> SNAASGSALIFDEEMSRYKLLWTDPACEIEVPERLTVSYEALRTHGLAQRCKAVPVRQATEQEILLAHSEEYLEAVKQTPGMNVEELMAFSKKYNDVYFHQNIYHCAKLAAGATLQLVDSVMKREVRNGMALVRPPGHHSQRSAANGFCVFNNVAFAALYAKKNYNLNRILIVDWDVHHGQGIQYCFEEDPSVLYFSWHRYEHQSFWPNLPESDYSSVGKGKGSGFNINLPWNKVGMTNSDYLAAFFHVLLPVAYEFDPELVIVSAGFDSAIGDPEGEMCALPEIFAHLTHLLMPLAAGKMCVVLEGGFNLTSLGQSVCQTVHSLLGDPTPRISGLGTACDSALESIQNVRNVQSSYWSSFKHLAQSETNPKRPRLDATNGGPKESSEPASESNPKKTAQDIVWPEPLKRMPASVRTVVVPPPGVELTLPKNCQHSGDISESTAKEVQRIRDKHFHDLTDQNILRSLGNIISVLDRMMRSDEVCNGCVVVSDLSVSVQCALQHALTEPAERVLVVYVGDGELPVKTNDGKVFLVQICTKETEDKCVNRLTLCLREGESLTAGFMQALLGLILPVAYEFNPALVLGIVEETAAKTRLMRVWGHMTCLIQGLARGRMLTLLQGYDKDLLELTVSALSGASISPLGPLRAPKPEDVEMMEKQRQRLQERWGLLRCTVSESW

Here we report enzymological studies conclusively demonstrating that HDAC10 is a robust PDAC and a poor lysine deacetylase. Therefore, HDAC6 is clearly an acetyllysine deacetylase and HDAC10 is an N8-acetylspermidine deacetylase. In addition, we report the 2.85-Å resolution crystal structure of HDAC10 complexed with a polyamine transition state analogue inhibitor. This structure reveals that the conserved glutamate gatekeeper and a sterically constricted active site confer specificity for N8-acetylspermidine hydrolysis and disfavour acetyllysine hydrolysis. Given that HDAC10 is a PDAC with catalytic specificity for the hydrolysis of N8-acetylspermidine to yield spermidine and acetate, it is possible that the functions of HDAC10 and spermidine in autophagy are linked.

To provide a molecular foundation for understanding the PDAC activity of HDAC10, we determined the 2.85 Å-resolution crystal structure of Y307F zHDAC10 complexed with the trifluoromethylketone inhibitor 7-[(3-aminopropyl)amino]-1,1,1-trifluoroheptan-2-one (AAT), which mimics N8-acetylspermidine24. This inhibitor binds as a transition state analogue with Ki=0.7±0.2 μM. We treated full-length zHDAC10 with trypsin to yield a heterodimeric complex, designated zHDAC10Δ, comprising the amino-terminal PDAC domain and the C-terminal pseudo-deacetylase (ΨDAC) domain. The proteolytically nicked zHDAC10Δ construct retains substantial catalytic activity. Both proteolysis and the introduction of the deactivating Y307F mutation facilitated crystallization. The crystal structure of the Y307F zHDAC10Δ–AAT complex revealed an overall butterfly-like architecture with a pseudo-two-fold symmetry axis perpendicular to several α-helices defining the PDAC-ΨDAC domain interface. Interdomain interactions were mediated by α-helices αF and αG, loop LH (which connects αH1 and αH2) and the C-terminal tail of each domain, burying ∼1,700 Å2 surface area. A close-up view of the active site tunnel revealed a canonical HDAC active site at the base of the tunnel, with AAT binding in an extended conformation. The trifluoroketone moiety of AAT formed a gem-diolate, making asymmetric coordination interactions with Zn2+ (O1-Zn2+ and O2-Zn2+ coordination distances of 2.1 and 2.5 Å, respectively); hydroxyl group O2 also hydrogen bonded with H136 and H137. On one side of the active site, gatekeeper E274 was close (3.7 Å) to the N4 atom of AAT. Opposite E274, there was an additional constriction contributing to PDAC specificity: a unique one-turn 310-helix ηA2 (P23ACE) resulting from a two-residue insertion plus a two-residue mutation in the L1 loop relative to zHDAC6, effectively lengthening the narrow active site tunnel by ∼5 Å.>NVQFSNQDGALGEPANYT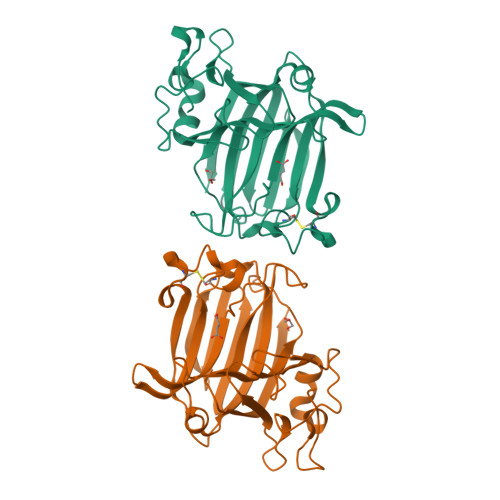QFQHVLTESELQISDAEGKKGNKEYFALDGNFTGIVNQYFYVDKKSEALVFKMKNDHLRNEVRVHKNFRTDLPNKLYTLSAEVEIIDPVASMKNSNSKQNEITFLQVHNKGLDNQGTHNVPHPLLRVVWKEDANSVKGHFWAMVKNNAVICKGSFGKKNKDKEMCKADVAYKKYDLGKAPLNKATAFDITVGNKQLIIDVDGKRLVEHDIDYWRHLLSYFKAGVYNQFTNGMSEAHFNKLEYKALE[2x]(2S)-1-[(2S)-6-amino-2-({[(2S,3S,4R,5S,6S)-3,4,5-trihydroxy-6-methyltetrahydro-2H-pyran-2-yl]acetyl}amino)hexanoyl]-N-[(1S)-1-carbamoyl-3-methylbutyl]pyrrolidine-2-carboxamide 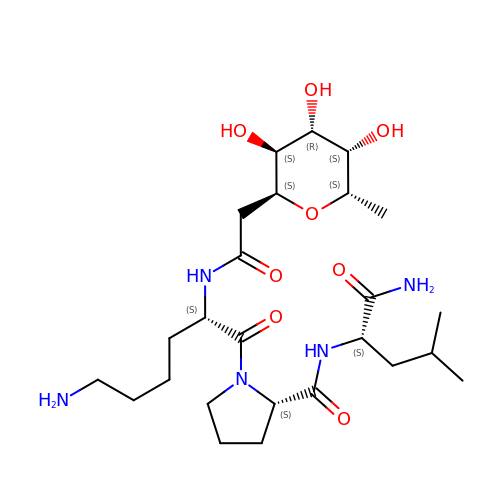| C25 H45 N5 O8 | GOIFOXKHMWJIPQ-OXQNIBOTSA-N> ATLDSWLSNEATVARTAILNNIGADGAWVSGADSGIVVASPSTDNPDYFYTWTRDSGLVLKTLVDLFRNGDTSLLSTIENYISAQAIVQGISNPSGDLSSGAGLGEPKFNVDETAYTGSWGRPQRDGPALRATAMIGFGQWLLDNGYTSTATDIVWPLVRNDLSYVAQ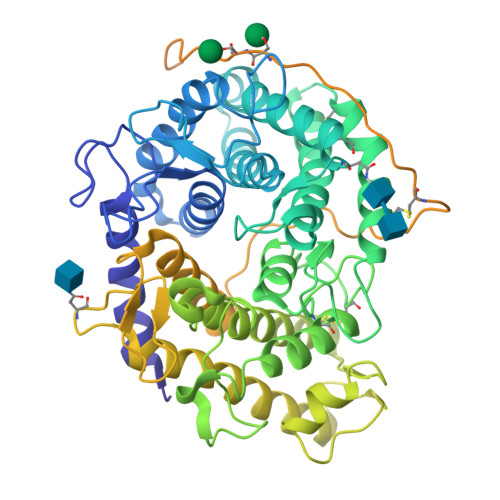YWNQTGYDLWEEVNGSSFFTIAVQHRALVEGSAFATAVGSSCSWCDSQAPEILCYLQSFWTGSFILANFDSSRSGKDANTLLGSIHTFDPEAACDDSTFQPCSPRALANHKEVVDSFRSIYTLNDGLSDSEAVAVGRYPEDTYYNGNPWFLCTLAAAEQLYDALYQWDKQGSLEVTDVSLDFFKALYSDAATGTYSSSSSTYSSIVDAVKTFADGFVSIVETHAASNGSMSEQYDKSDGEQLSARDLTWSYAALLTANNRRNSVVPASWGETSASSVPGTCAATSAIGTYSSVTVTSWPSIVATGGTTTTATPTGSGSVTSTSKTTATASKTSTSTSSTSCTTPTAVAVTFDLTATTTYGENIYLVGSISQLGDWETSDGIALSADKYTSSDPLWYVTVTLPAGESFEYKFIRIESDDSVEWESDPNREYTVPQACGTSTATVTDTWR> MYKQRFLELWEELHDPSNGYFSSHGIPYHAVETLIVEAPDYGHLTTSEAMSYYLWLEALYGKFTGDFSYFMKAWETIEKYMIPDSTEQPGMSSYNPNSPATYADEYEDPSYYPSELKFDTVRVGSDPVHNDLVSAYGPNMYLMHWLMDVDNWYGFGTGTRATFINTFQRGEQESTWETIPHPSIEEFKYGGPNGFLDLFTKDRSYAKQWRYTNAPDAEGRAIQATYWANQWAKEHGVNLSQYVKKASRMGDFL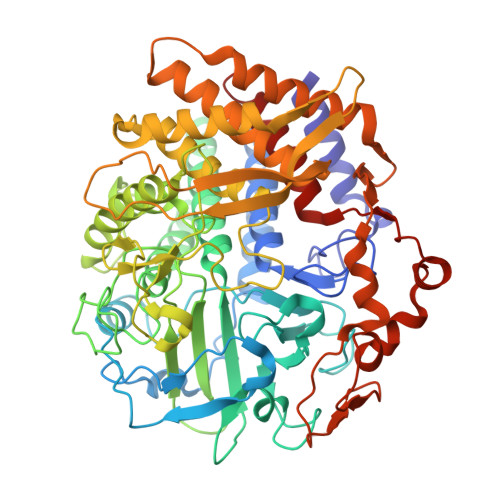RNDMFDKYFMKIGAQDKTPATGYDSAHYLMAWYTAWGGGIGASWAWKIGCSHAHAGYQNPMTAWILANDPEFKPESPNGANDWAKSLERQLEFYQWLQSAEGGIAGGATNSWNGRYEKYPAGTSTFYGMAYVPHPVYADPGSNQWFGFQAWSMQRVMEYYLETGDSSVKNLIKKWVDWVMSEIKLYDDGTFAIPSDLEWSGQPDTWTGTYTGNPNLHVRVTSYGTDLGVAGSLANALATYAAATERWEGKLDTKARDMAAELLDRMWNLYRDDKGLSAPETREDYVRFFEQEVYVPQGWSGTMPNGDRIEPGVTFLDIRSKYLNDPDYPKLQQAYNEGKAPVFNYHRFWAQCDIAIANGLYSILF[4-[(4-methyl-1,4-diazepan-1-yl)methyl]phenyl]methanamine 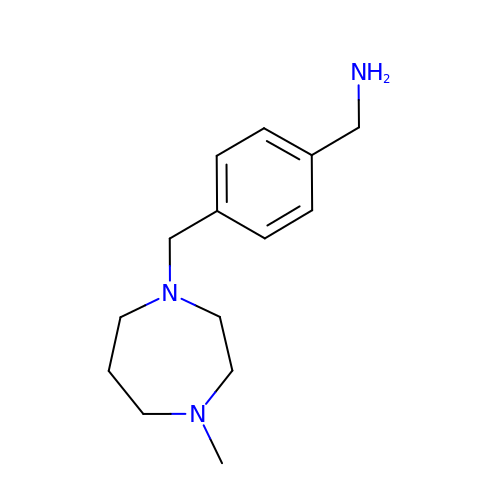| C14 H23 N3 | AQLZGQUKWNQYPH-UHFFFAOYSA-N> MDQENFHGSSLPQQLQNLHIQPQQASPNPVQTGFAPRRHYNNLVGLGNGNAVSGSPVKGAPLGQRHVKLKKEKISAQVAQLSQPGQLQLSDVGDPALAGGSGLQGGVGLMGVILPSDEALKFVSETDANGLAMKTPVSILQELLSRRGITPGYELVQIEGAIHEPTFRFRVSFKDKDTPFTAMGAGRSKKEAKHAAARALIDKLIGAQLPESPSSSAGPSVTGLTVAGSGGDGNANATGGGDASDKTVGNPIGWLQEMC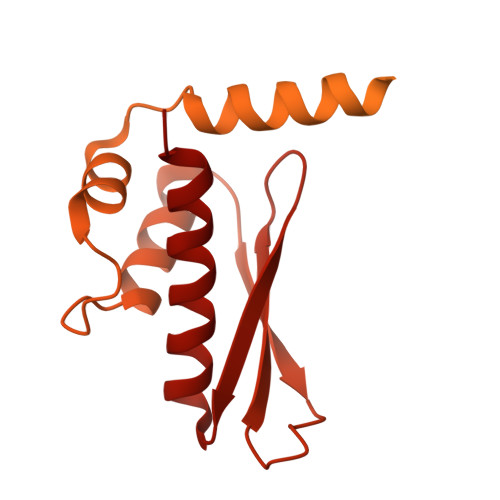MQRRWPPPSYETETEVGLPHERLFTIACSILNYREMGKGKSKKIAKRLAAHRMWMRLQETPIDSGKISDSICGELEGEPRSSENYYGELKDISVPTLTTQHSNKVSQFHKTLKNATGKKLLKLQKTCLKNNKIDYIKLLGEIATENQFEVTYVDIEEKTFSGQFQCLVQLSTLPVGVCHGSGPTAADAQRHAAQNALEYLKIMTKK1-{[1,3-dimethyl-7-(3-methylbutyl)-2,6-dioxo-2,3,6,7-tetrahydro-1H-purin-8-yl]methyl}piperidine-4-carboxamide | C19 H30 N6 O3 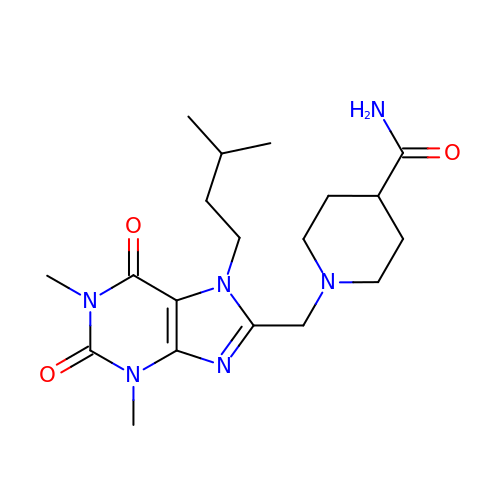| IOCDTSBNIYANHP-UHFFFAOYSA-N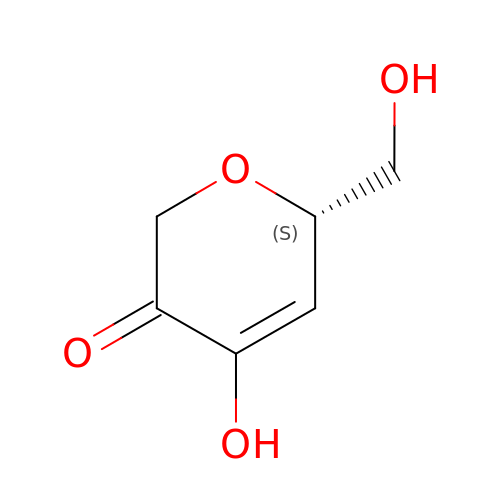Ascopyrone M | C6 H8 O4 | XUKJGZOHRVCEJL-BYPYZUCNSA-N>HSHRDFQPVLHLVALNAPLSGGMRGIRGADFQCFQQARAVGLAGTFRAFLSSRLQDLYSIVRRADRAAVPIVNLKDELLFPSWEALFSGSEGPLKPGARIFSFDGKDVLRHPTWPQKSVWHGSDPNGRRLTESYCETWRTEAPSATGQASSLLGGRLLGQSAASCHHAYIVL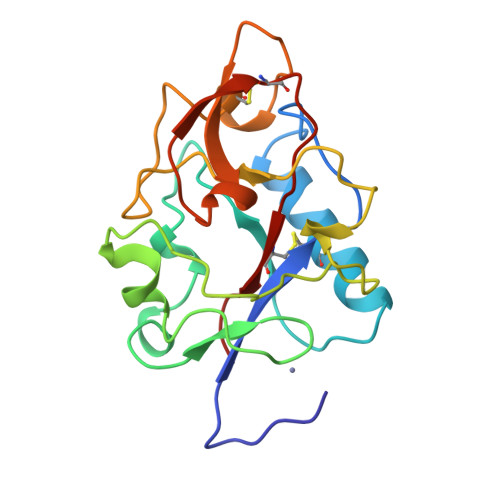CIENSF[4x]>GSHMWDTANNPLYKEA[4x];>[4x]PVQLNLLYVQARDDILNGSHPVSFDKACEFAGYQCQIQFGPHNEQKHKPGFLELKDFLPKEYIKQKGERKIFMAHKNCGNMSEIEAKVRYVK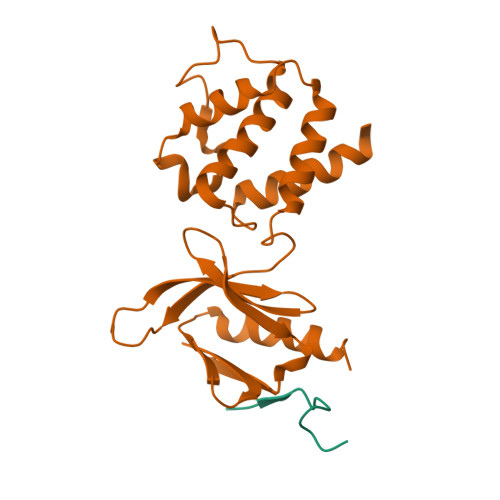LARSLKTYGVSFFLVKEKMKGKNKLVPRLLGITKECVMRVDEKTKEVIQEWSLTNIKRWAASPKSFTLDFGDYQDGYYSVQTTEGEQIAQLIAGYIDIIL> MEEDIACVKDLVSKYLANNERLSRQKLAFLVQTEPRMLLMEGLKLLSLCIEVDSCNANGCEHNSEDKSVERILHDHGVLTPSLCFVVPDGYKLTGNVLILLECFVRSSPANFEQKYVEDFKKLEQLKEDLKSVDINLIPLIDGRTSFYNEQIPDWVNDKLRDTLFSLLKYAQESNSLFEESEYSRLCESLSMTSGRLSGVESLNALLDNRSNHYEEVIASCHQGINNKLTAHEVKLQIEEEYQVFRNRLRKGEIEGQFLKVEKNQLLNEFNNLYADKVAEKDSVEHLTHQFKRASPILRFLYANISKGDNGEGNLIIGECQMQCWRSFLNKVKSMRILNTRRKLLLIFDALILLASKHDQVRKKPLRGWLGTCFVSVNDRLVSLESTKKDLKKWVERRQQVERSRTMQSFQCPSKNQILNSIFQKTISKATTALRDVGISVDHYKIDMEVICPDGYDLIMDFDVSGVTPTISYQRSEEEAFPYIMGDVDLLKTTDLERLSSLSLALVNSMKTSSTVKLRQNEFGPARYQVVKCKEAYCQEFSLGETEFQLIYQKTGECSKCYAINDNRVGEVCSFYADPKRYFPAIFSAEVLQTTVSTMISWIEDCNELEEQLDKIRSLTKMILILILAHPSKRSQKLLQNLRYFIMAYVSDYYHKDLIDKVREELITDVEFLLYRLLRTLMGLVLSEDVKSMMTNRFKFILNISYMCHFITKETPDRLTDQIKCFEKFLEPKVKFGHVSINPADTATEEELDDMVYNAKKFLSKGGCTSAKGPSYKKPGVSKKYLSLLTSSFNNGSLFKEREVKKEIKDPLITSGCATALDLASNKSVVVNKYTDGSRVLNYDFNKLTALAVSQLTEVFSRKGKHLLNKQDYEYKVQQAMSNLVLGSKQHKGDADEADLDEILLDGGASTYFNQLKETVEKIVDQYREPVKMGSGSNDGDQPSINDLDEIVSNKFYIRLIKGELSNHMVEDFDHDVLPDKFYEEFCDAVYENSKL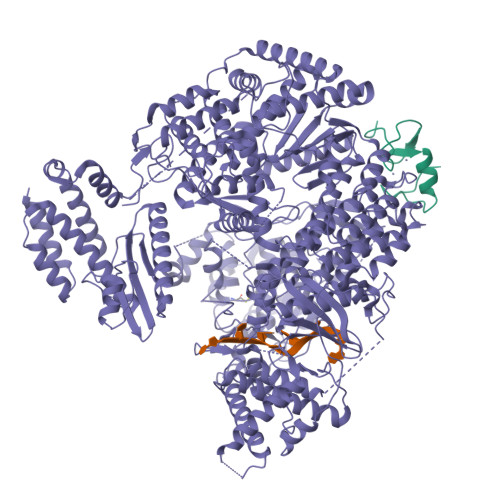KEKYFYCGHMSQCPIGELTKAVSTRTYLDHEYFQCFKSILLIMNANALMGKYTHYKSRNLNFKFDMGKLSDDARISERESNSEALSKALSLTNCTTAMLKNLCFYSQESPQSYNSVGPDTGRLKFSLSYKEQVGGNRELYIGDLRTKMFTRLIEDYFEALSSQLSGSCLNNEKEFENAILSMKLNVSMAHVSYSMDHSKWGPMMCPFLFLTVLQNLIFLSKDLQADIKGRDYLSTLLMWHMHKMVEIPFNVVSAMMKSFIKAQLGLRKKTKQSITEDFFYSNFQIGVVPSHISSILDMGQGILHNTSDFYALITERFINYAISCVCGGTIDAYTSSDDQISLFDQTLTELLHRDPEEFRALMEFHYYMSDQLNKFVSPKSVIGRFVAEFKSRFFVWGDEVPLLTKFVAAALHNIKCKEPHQLAETIDTIVDQSVANGVPVHLCNLIQIRTLSLLQYARYPIDPFLLNCETDVRDWVDGNRSYRIMRQIEGLIPDACSKIRSMLRRLYNRLKTGQLHEEFTTNYLSSEHLSSLKNLCELLGVEPPSESDLEYSWLNLAAHHPLRMVLRQKIIYSGAVNLDDEKIPTIVKTIQNKLSSTFTRGAQKLLSEAINKSAFQSSIASGFVGLCRTLGSKCVRGPNKENLYIKSIQSLITGTQGIELLTNSIGVQYWRVPLGLRNKSESVVSYFRPLLWDYMCISLSTAIELGAWVLGDPKTTKALDFFKHNPCDYFPLKPTASKLLEDRVGLNHIIHSLRRLYPSVFEKHILPFMSDLASTKMKWSPRIKFLDLCVALDVNCEALSLVSHIVKWKREEHYIVLSSELRFSHTRTHEPMVEERVVSTSDAVDNFMRQIYFESYVRPFVATTRTLGSFTWFPHRTSIPEGEGLHRLGPFSSFVEKVIHKGVERPMFKHDLMMGYAWIDFDIEPARFNQNQLIASGLVDSKFDSLEDFFDAVASLPTGSAKLSQTVRFRIKSQDASFRESFAIHLDYIGSMNQQAKYLVHDVTAMYSGAVSPCVLSDCWRLVLSGPTFKGKPVWYVDTEVINEFLVDTNQLGHVTPVEVVVDMEKLQFAEYDFMLVGPCAEPVPLVVRRGGLWECEKKLASFTPVIQDQDLEMFVREVGDTSSDLLIRALSDMITDRLGLRMQWSGVDIVSTLRAAAPGNAEVLSAVLEVVDNWVEFKGYALCYSKSRGRVMVQSSSGKLRLKGRTCEELTEGGEHVEDIE;> MGNKQVKAPEARNSPRASLIPDATHLGPQFCKSCWAENKGLVECNNHYLCLNCLTLLLGVSSRCPICKMPLPTRLRPSAAPTAPPAEAGDNTRPPPYSP>[2x]MSAERILVTGGAGFIGSHLVDALLAKGYAVRVLDDLSTGKVGNLPMGDAGLELLVGDAADAALLADAVQGCDAVVHLAAVASVQASVEDPVATHQSNFIATLRLCEAMTAAGIRRVVFASSAAV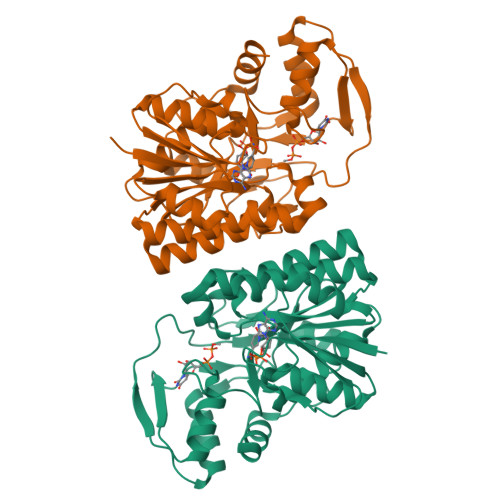YGNNGEGTPIAEDTPKSPLTPYAADKLASEYYLDFYRRQHGLEPVILRFFNIFGPRQDPSSPYSGVISIFSERAKAGRPITLFGDGGQTRDFVYVADLVKILVQGLESPAPAADATNVGLGGVTTLNDLIGALQQISGKPLQVSHGATRSGDIRHSKADNRRLRERFDLGTPSSLAEGLERLYRSL> MSLFVVNAPGHEGQLKEQLIVAHKRRPLLATAWVNPPSVLITNSEGEVLTQVADPPGSTGRTHQPTALTWHPNEELLVIGWSNGEMSLWSMPSVSSLALGEDYTTAAARSAVQLIAAKAATQSSAEGATREHASGAVVASEWSTRGLYLVSASQQRHVVMWMLEKIPAETSVTFKLKPLWSVQSREPVARIIHVPSKASHPSTAFKLNNGATAAAAAEGGDDDISFLLADGGTSVTAINEDQQLFPCVTQQEQIASVLYDAATRTLVTLTTTSMIEVYAVGEDIKGTSTLRRKLSAPATTPTVSTTTGERIAMSMVWASPGVVAFGSGDDRLRILDLSSGSLDVLLLPQPDLHVSSLATFAAKGTMIVGTVEGFLVVFQHHAASLLTSRHVSVARETVTSSSPFAPAATEASQWEAMTVHQVGKCVDRVVLTALGDVALCCGGSELQVLHEIIRKRAWDGVAAATQISSDMVVIESITGCQCLLQNKGNVHGVSIAFPNIALWNGSQIDFYMIDEATSEITFINFVLTTSPAFAIHREGLIYVKGNRIVFETMQLAPIAQMTFTESEGVPVIMDIMNDYLVVVSSKNYLRLARISTRDLQQLGPARPLTFPSILQPDAVEASSGASEMTPFVEDISTLEVSVSGARVNAQGRRVALMSTLGPLALPDTRIWVYDSDTDKMSFFDFGSRNEIPNSVYWNTPEPNTTTVGEFEYILLACETYQIHMDDKKSASEEAESPKACTDTTNDGNKIADHPVGQENLPEALPDMENYAEKKAELEDARRESVGTTNYVSQRPHNIVTFFATHDGLVLQNFAPLRRYQICLVGLTIPDFLLASVKINGDPNNAEDYVIEQKRLRDFEGLKSDKDVAVREALMKFSYYATIG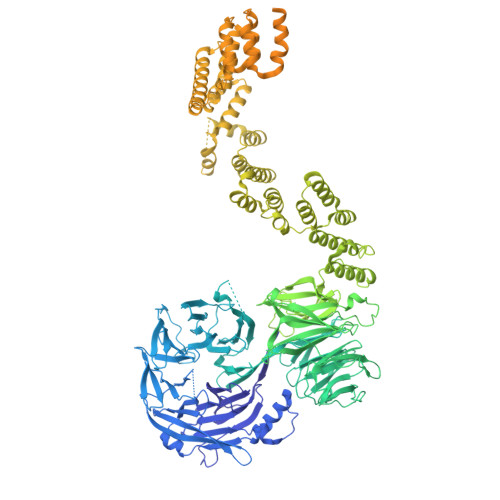NMDEAYRCVKSIKNPAAWQGLARLCVTSGRLDVAAVCLATMEDCVAARALREAKEDYPDDQDVQLATLALGLSMTEEAVELLRKSKRYDLLTDVYMACGKFEHAQRHSERFDRARIRPVAYKYAQFMESLQNMDAAIMWYYNAKCASTDVPRIFFQTNRMHELRQLMMIQSQPPSPTAGDSAQRPQPGIGEQQSTFATIFPQNRELLLWWAQHSERRHNVQEALRFYNAGEDVYNIVRILCSLTPPKLDSALQLVNKEMDKAKMRFQQQQAFAATASARFGDDDHGEPDPVGSAYFVAQLYERQGDDQLALQYYQAAGAYRSGVRVAWKMEQYGVVANLAMKSSDERLMLETAMALEKHQAYDKAVQLYRRIGAVQCALDACVQGGLYETLHEVSAAFASGSTDPAVFLGMADHFQSESDYQKAVEMLLFAKHFEEALKLCETQNATLTEEMAESMTSNIGELSMEERQAVLRRVAHIAKDQGRWSLACKKYTQAGDRVKAMRMLMRGGETEKVIFFANHSRNVEIYTMAANFLQSQNWSADANIYKSIVLFYTKAKAWMNLLAFYESCAQLHIDENRNYPEALRALEDCIAMAESVRGGKANIEMEKVEQLKQRVEILKAFVKAQKTVDSMVVAERGSVAEKAKADSVIACCSGLIKRSRPSSPDHSLIQDALRIGDVFALMVRFYFDKLGEPHNALKVMESMPKHGADPQLFIEADYMERVCQANGKSLANVLPGGIATEAPGAVWEGARKFSTDTRRSSVIDEVDRVV cGAS has emerged to be an essential protein for the innate immune response to cytosolic DNA given its activation of Sting by the production of cGAMP. The generation of cGAMP by cGAS requires that the enzyme bind to dsDNA and use its two substrates, ATP and GTP, to generate the cyclic dinucleotide. Our previous structural studies have shown that upon dsDNA binding, cGAS is activated through conformational transitions resulting in the formation of a catalytically competent and accessible nucleotide-binding pocket for generation of cGAMP14. Here, we report the discovery and characterization of a class of compounds that binds to the catalytic pocket of cGAS and inhibits its dsDNA-stimulated activity.

Using an in vitro mass-spectrometry based high-throughput compound screen, we initially identified RU.365 and its benzothiazole analog RU.332 as inhibitors of the dsDNA-induced enzymatic activity of cGAS. The only difference between RU.365 and RU.332 is the substitution of the benzimidazole ring with a benzothiazole ring; the two bound inhibitors can be superimposed very well with each other. We can distinguish S from N of the benzothiazole ring by checking the Fo-Fc map during refinement. The sulfane group is facing the aromatic/hydrophobic surface of the binding pocket, while the remaining methanamine group is pointing into the solvent region. We tested analogs with targeted substitutions in groups that can function as H-bond donors or acceptors since we previously observed that replacing the 1-N benzimidazole’s nitrogen by sulfur (RU.332) did not change the potency of cGAS inhibition, whereas ring conversion from isobenzofuranone to isoindolinone (RU320465) abolished inhibitory activity. To our surprise, by superposing the structures of inhibitor complexes with the structure of cGAS in free state, we found that RU.365/RU.332/RU.521 could also fit the “smaller active site” of apo-cGAS in the dsDNA-free state without notable steric effects. RU.332 and RU.521 show similar superposition results to that of RU. The above comparison suggests that RU.365/RU.332/RU.521 could potentially inhibit every catalytic step (substrate binding, intermediate and product formation) of cGAS, or could displace substrates from the catalytic pocket. The cellular IC50 value for RU.365 (4.98 µM) was approximately twofold lower than RU.332 (13.60 µM). We found that RU.365 led to increased Il-6 messenger RNA (mRNA) expression in cells activated by Pam3CSK4, poly(I:C), or LPS; none of the compounds caused reporter activation on their own. RU.332 inhibited the activation of cells by most of the immunogenic ligands tested.

> SPDKLKKVLDKLRLKRKDISEAAETVNKVVERLLRRMQKRESEFKGVEQLNTGSYYEHVKISAPNEFDVMFKLEVPRIELQEYYETGAFYLVKFKRIPRGNPLSHFLEGEVLSATKMLSKFRKIIKEEVKEIKDIDVSVEKEKPGSPAVTLLIRNPEEISVDIILALESKGSWPISTKEGLPIQGWLGTKVRTNLRREPFYLVPKNAKDGNSFQGETWRLSFSHTEKYILNNHGIEKTCCESSGAKCCRKECLKLMKYLLEQLKKEFQELDAFCSYHVKTAIFHMWTQDPQDSQWDPRNLSSCFDKLLAFFLECLRTEKLDHYFIPKFNLFSQELIDRKSKEFLSKKIEYERNNGFPIFDKL> GSHMALAKRVVHFDYDSSDLSTEDYQTLQAHAQFLMANANSKVALTGHTDERGTREYNMALGERRAKAVQNYLITSGVNPQQLEAVSYGKEAPVNPGHDE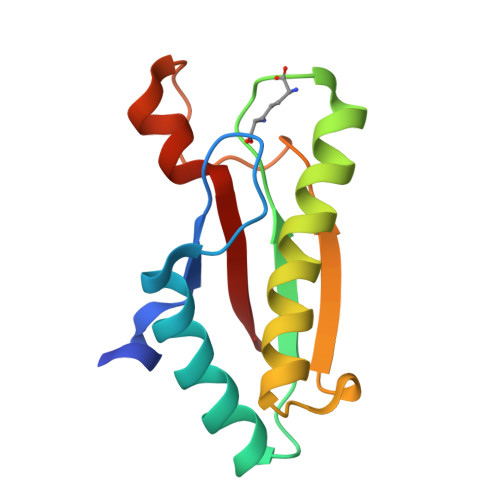SAWKENRRVEINYE>GHMAVPDDDDDDDNSNDESEYESSQMDSEKNKGSIKNSKNVVIYADGVYDMLHLGHMKQLEQAKKLFENTTLIVGVTSDNETKLFKGQVVQTLEERTETLKHIRWVDEIISPCPWVVTPEFLEKYKIDYVAHDDIPYANNQKEDIYAWLKRAGKFKATQRTEGVSTTDLIVRILKNYEDY[6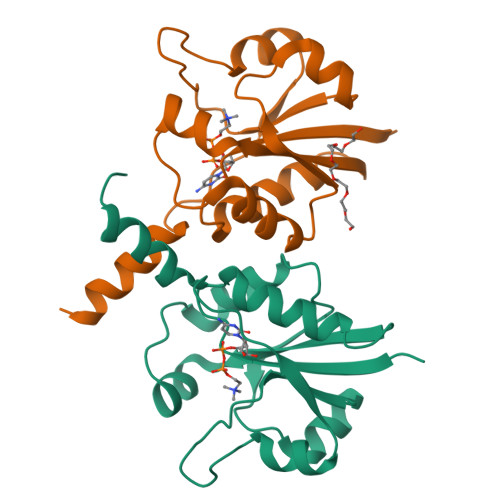x]> MTKKVGLLVMAYGTPYKDEDIERYYTDIRHGHKPSEEMIADLRGRYHAIGGLSPLAKITEAQAYGLEKALNDSQDEVEFKAYIGLKHIEPFIEDAVEAMHKDGIEEAISIVLAPHYSSFSVEAYNKRAKEAADKLGGPRINAINDWYKQPKFIQMWADRINETAKQIPADELLDTVLIVSAHSLPEKIKQHNDPYPNQLQETADFIFEKVVVPHYALGWQSEGKTGEPWLGPDVQDLTRELYGREKYKHFIYTPVGFVAEHLEVLYDNDYECKVVTDEVGAAYHRPPMPNSDPEFLEVLRTVVWEKYSN

Coproporphyrin ferrochelatase (CpfC) in the CPD heme biosynthesis pathway incorporates ferrous iron into coproporphyrin III (cpIII) to give coproheme, which is eventually decarboxylated to yield heme b by the coproheme decarboxylase enzyme in the final step of this biosynthetic process (Dailey et al., 2017; Dailey & Gerdes, 2015; Layer, 2021). Understanding structure–function relationships of key enzymes, such as ferrochelatase, is an essential precondition for the design of new inhibitors for antibiotic‐resistant pathogens, like Listeria monocytogenes. LmCpfC crystals in complex with cpIII were soaked with a ferrous iron solution and flash‐vitrified after 2, 3, and 4 min, to obtain snapshots of the enzymatic reaction during iron insertion into the porphyrin macrocycle. We report three crystal structures showing different iron content during metalation in LmCpfC, identifying the presence and defining the extent of the porphyrin distortions during iron insertion.

In the "68% Fe" structure (resolution 2.1 Å) the best refinement solution was identified with the ferrous iron being present at 68% occupancy. Interestingly, in the “68% Fe” structure, we observe a continuous electron density from the distal histidine (H182) to the proximal tyrosine (Y12). Ring A with the substituent p2 exhibits the highest distortion in the “34% Fe” structure (+12.6°), +9.2° in the cpIII structure and lowered values for the “24% Fe” (+4.8°), and the “68% Fe” (+1.9°) structures; in ring B (p4) the angle is altered the most in the analyzed samples (−13.4°, −10.5°, −11.4°, and −6.7°) as a function of the site occupancy by Fe ions, exhibiting a high degree of distortion compared to the coproheme structure. The measured change of angles throughout the ferrous iron insertion process at the site of p7 at pyrrole ring D is also peculiar: the rings in the substrate‐ and product‐bound states overlap well for all structures besides the “24% Fe” structure (−2.1° in the cpIII‐structure, −1.6° in the "68% Fe" structure, and −1.4° in the "34% Fe" structure). In the “24% iron occupancy” and in the coproheme‐bound structures, the guanidinium group points toward p7, while in the “68% iron occupancy” structure, being in a split conformation, partially points outwards since one conformation is 5.4 Å from p7. The residue points toward p7 in the “24% Fe”, “34% Fe”, and in the coproheme‐complex structures, but points away (5.4 Å) in the “68% Fe” structure. Nevertheless, a definitive conclusion cannot be drawn as the ionic radius of the ferrous iron in the “24% Fe”, “34% Fe”, and “68% Fe” structures is larger than the ionic radius of the ferric ion in the coproheme product and would result in an out‐of‐plane position regardless of the side from which it is approaching.2-[(3-fluorophenyl)methyl]-1lambda~6~,2-thiazolidine-1,1-dione | C10 H12 F N O2 S | 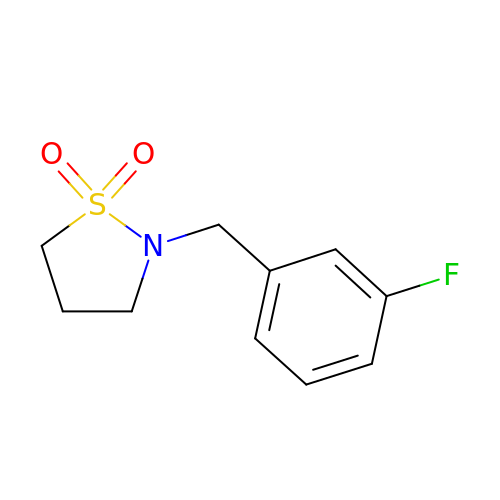RVDJKNWVTKGWCE-UHFFFAOYSA-N> MASAHIALELDKTKVKVGDVIVATVKAKNMTSMAGIQVNIKYDPEVLQAIDPATGKPFTKETLLVDPELLSNREYNPLLTAVNDINSGIINYASCYVYWDSYRESGVSESTGIIGKVGFKVLKAANTTVKLEETRFTPNSIDGTLVIDWYGQQIVGYKVIQPDLEHHHHHH;> MNKPVIEGYKVSGYILPDFSFDATVAPLVKAGFKVEIVGTELYAVTDANGYFEITGVPANASGYTLKISRATYLDRVIANVVVTGDTSVSTSQAPIMMWVGKIVKDNSINLLDVAEVIRCFNATKGSANYVEELDINRNGAINMQDIMIVHKHFGATSSDYDAQ

In addition, cellulosomes are central elements for the production of readily available sugars in the gastrointestinal tract of a variety of mammals4. It is now well established that a wide array of highly ordered protein-protein interactions involving dockerin and cohesin modules (defined herein as Doc and Coh, respectively) mediate both cellulosome assembly and cellulosome cell-surface attachment. Primary scaffoldins, in addition to containing multiple type-I Cohs, have a divergent type-II Doc that binds to type-II Cohs located in cell-surface anchoring scaffoldins, providing a mechanism to tether the cellulosome to the bacterial cell envelope. In addition to ScaA, inspection of C. thermocellum genome revealed the presence of an ORF (Cthe_1806) encoding a protein comprising 2177 amino acids and containing a putative type-II Doc, which was termed CipB. Type-II Docs of primary scaffoldins ScaA and CipB in C. thermocellum possess two distinct Coh-binding surfaces that recognize different Coh partners.

In ScaF Coh this residue is replaced by a Ser, and the β-flap is placed further away from the Coh-binding interface. This comparison indicates that the side chain of Phe136 in the ScaC2 Coh would clash with the side chain of Asn122 in ScaA Doc, strongly suggesting that the ScaA Doc is unable to bind Coh ScaC2 in this orientation. However, considering the inherent symmetry allowed by the interaction of two Doc helices to the Coh platform, it is possible that, if rotated by 180°, the ScaA Doc would be better positioned to bind ScaC2 Coh, a hypothesis that was further explored below. Thus, in order to probe the mechanism by which CipB XDoc binds to ScaF and ScaA XDoc recognises ScaC2, the crystal structures of ScaF XDoc in complex with ScaC2 Coh (CtCohScaC2-XDocScaA) and CipB XDoc bound to ScaF (CtCohScaF-XDocCipB) were solved. Strikingly, the data revealed that the two Docs bound ScaF and ScaC2 in different orientations. In contrast, ScaC2 Coh recognized ScaA XDoc, predominantly through helix 1 and CipB XDoc through helix 3. When the two complexes comprising ScaC2 Coh were overlaid (CtCohScaC2-XDocScaA and CtCohScaC2-XDocCipB), it was evident that the XDoc modules were in reverse orientations highlighted by the X-modules, which were positioned in opposite directions. Both ScaC2 Coh and the type-II Docs display a high degree of similarity when these protein modules were independently compared, which is reflected by the low r.m.s.d values (0.5 Å for 160 Cα atoms of the Coh alone and 1.1 Å for 54 Cα atoms of the Doc module). Although the nature of the hydrophobic interactions is almost indistinguishable, the ScaA Doc, which binds ScaC2 predominantly through helix 1, makes an extra hydrogen bond to Phe136 through Ser108. Steric constraints do not accommodate Asn158/Asn122 in binding ScaC2 and thus these residues are replaced by Gly125/Gly155 when binding to this Coh.4-{3-[(4-methyl-1-benzothiophen-3-yl)methyl]-2-oxo-2,3-dihydro-1H-benzimidazol-1-yl}butanoic acid | C21 H20 N2 O3 S | 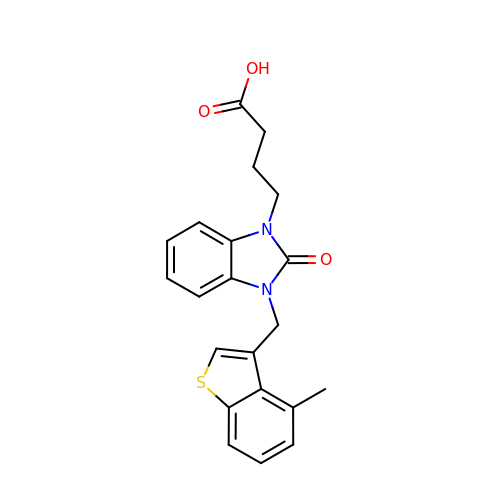WYBNXPWKJQJMLG-UHFFFAOYSA-N>[2x]MPPLSLLIKPASSGCNLKCTYCFYHSLSDNRNVKSYGIMRDEVLESMVKRVLNEANGHCSFAFQGGEPTLAGLEFFEKLMELQRKHNYKNLKIYNSLQTNGTLIDESWAKFLSENKFLVGLSMDGPKEIHNLNRKDCCGLDTFSKVERAAELFKKYKVEFNILCVVTSNTARHVNKVYKYFKEKDFKFLQFINCL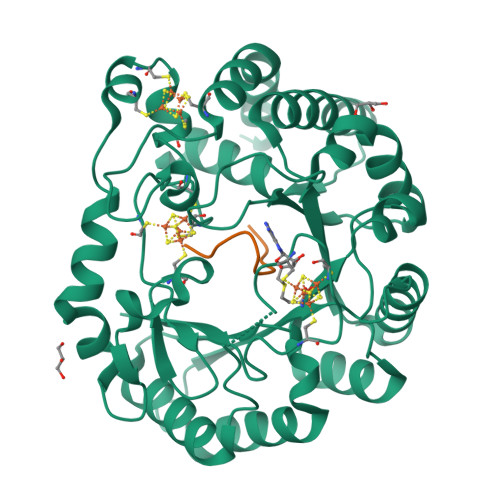DPLYEEKGKYNYSLKPKDYTKFLKNLFDFWYEDFLNGNRVSIRYFDGLLETILLGKSSSCGMNGTCTCQFVVESDGSVYPCDFYVLDKWRLGNIQDMTMKELFETNKNHEFIKLSFKVHEECKKCKWFRLCKGGCRRCRDSKEDSALELNYYCQSYKEFFEYAFPRLINVANNIK;>YTAVPSCIPSRASILTGM[2x]> MGAQVSSQKVGA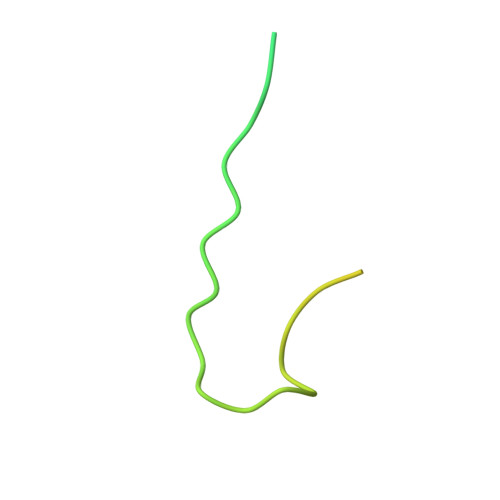HENSNRAYGGSTINYTTINYYKDSASNAASKQDYSQDPSKFTEPLKDVLIKTAPALN>[4x]MAEQVALSRTQVCGILREELFQGDAFHQSDTHIFIIMGASGDLAKKKIYPTIWWLFRDGLLPENTFIVGYARSRLTVADIRKQSEPFFKATPEEKLKLEDFFARNSYVAGQYDDAASYQRLNSHMNALHLGSQANRLFYLALPPTVYEAVTKNIHESCMSQIGWNRIIVEKPFGRDLQSSDRLSNHISSLFREDQIYRINHYLGKEMVQNLMVLRFANRIFGPIWNRDNIACVILTFKEPFGTEGRGGYFDEFGIIRDVMQNHLLQMLCLVAMEKPASTNSDDVRDEKVKVLKCISEVQANNVVLGQYVGNPDGEGEATKGYLDDPTVPRGSTTATFAAVVLYVENERWDGVPFILRCGKALNERKAEVRLQFHDVAGDIFHQQCKRNELVIRVQ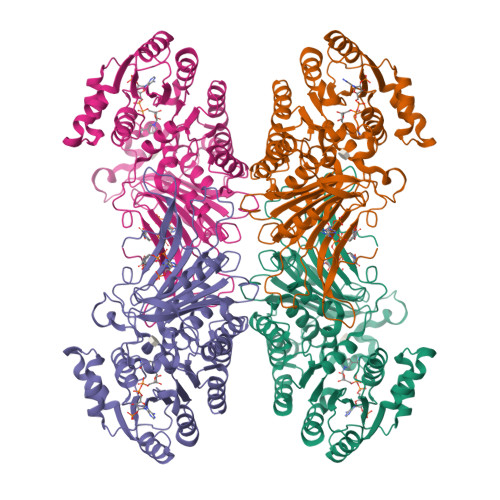PNEAVYTKMMTKKPGMFFNPEESELDLTYGNRYKNVKLPDAYERLILDVFCGSQMHFVRSDELREAWRIFTPLLHQIELEKPKPIPYIYGSRGPTEADELMKRVGFQYEGTYKWVNPHKLLEHHHHHH> MHTTLFFSNRT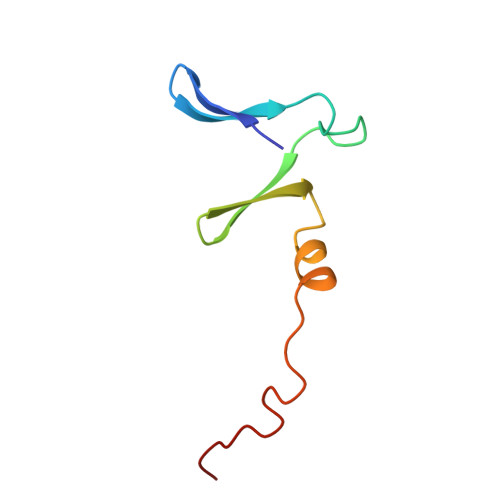QAVRLPKSISFPEDVKHVEIIAVGRSRIITPVGESWDSWFDGEGASTDFMSTREQPA>[2x]GHMSSEFQINEQVLACWS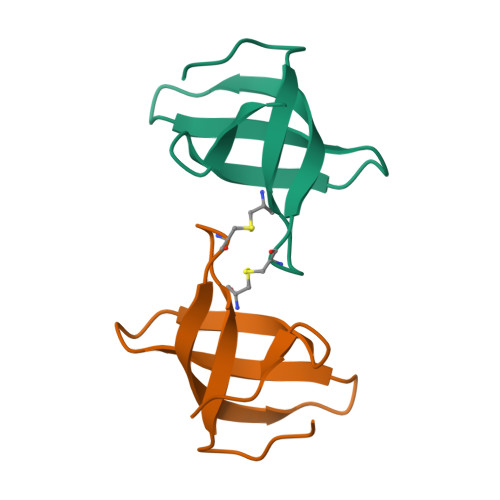DCRFYPAKVTAVNKDGTYTVKFYDGVVQTVKHIHVKAFSKDQNIVGNAR>[2x]NAKGNYCKRTPLYIDFKEIGWDSWIIAPPGYEAYECRGVCNYPLAEHLTPTKHAIIQALVHLKNSQKASK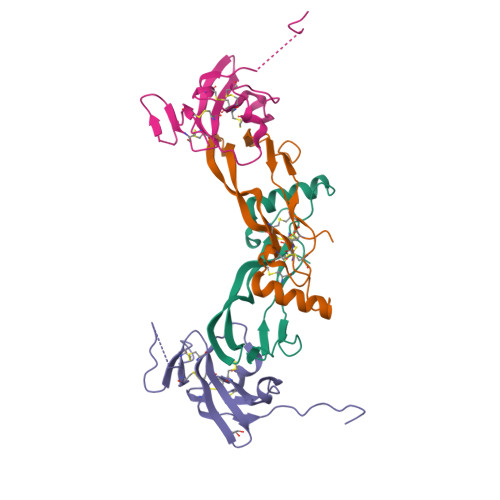ACCVPTKLEPISILYLDKGVVTYKFKYEGMAVSECGCR;>[2x]GSQNQERLCAFKDPYQQDLGIGESRISHENGTILCSKGSTCYGLWEKSKGDINLVKQGCWSHIGDPQECHYEECVVTTTPPSIQNGTYRFCCCSTDLCNVNFTENFPPPDTTPLSPPHSFNRDET>[2x]GGLEKDFLPLYFGWFLTKKSSETLRKAGQVFLEELGNHKAFKKELRHFISGDEPKEKLELVSYFGKRPPGVLHCTTKFCDYGKAAGAEEYAQQEVVKRSYGKAFKLSISALFVTPKTAGAQVVLTDQELQLWPSDLDKPSASEGLPPGSRAHVALGCAADVQPVQTGLDLLDILQQVKGGSQGEAVGELPRGKLYSLGKGRWMLSLTKKMEVKAIFTGYYG

2′,3′-cyclic nucleotide 3′-phosphodiesterase (CNPase) comprises 4% of total myelin protein in the central nervous system (CNS), being the most abundant CNS non-compact myelin protein4. CNPase consists of an N-terminal polynucleotide kinase-like domain10, a catalytic phosphodiesterase domain11, and a membrane-anchored C-terminal tail, which contains a cysteine residue that undergoes isoprenylation. The catalytic domain enables the rapid hydrolysis of nucleoside 2′,3′-cyclic phosphates to nucleoside 2′-phosphates. The CNPase catalytic site, lying in a groove between two lobes, has pseudo two-fold symmetry and contains two apposing His-X-Thr-X (X denotes a hydrophobic residue) motifs, characteristic for 2H phosphoesterases 113537.

In addition to the catalytic His mutants, near-complete catalytic inactivation is evident also in T232A, T311A, F235A, F235L, and Y168A. The inactivation by the T232A and T311A mutations was expected: threonine or serine is found in the catalytic motif in all 2H phosphoesterases, and in CNPcat, they are involved in all stages of catalysis, in achieving the correct substrate binding mode together with His230, His309, and the active-site water network.>[2x]MVL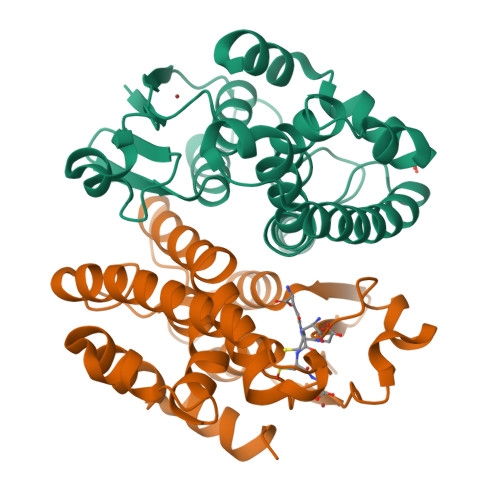KVYGPHFASPKRALVTLIEKGVAFETIPVDLMKGEHKQPAYLALQPFGTVPAVVDGDYKIFESRAVMRYVAEKYRSQGPDLLGKTVEDRGQVEQWLDVEATTYHPPLLNLTLHIMFASVMGFPSDEKLIKESEEKLAGVLDVYEAHLSKSKYLAGDFVSLADLAHLPFTDYLVGPIGKAYMIKDRKHVSAWWDDISSRPAWKETVAKYSFPA> MKHHHHHHMKQNSPLDEENLTQENQDRGTHVDRGLASANVDFAFSLYKQLVLKAPDKNVIFSPLSISTALAFLSLGAHNTTLTEILKGLKFNLTETSEAEIHQSFQHLLRTLNQSSDELQLSMGNAMFVKEQLSLLDRFTEDAKRLYGSEAFATDFQDSAAAKKLINDYVKNGTRGKITDLIKDLDSQTMMVLVNYIFFKAKFEMPFDPQDTHQSRFYLSKKKYVMVPMMSLHHLTIPYFRDEELSCTVVQLNYTGNASALFILPDQDKMEEVEAMLSQETLSRFFDSLEFREIGELYLPKFSISRDYNLNDILLQLGIEEAFTSKAD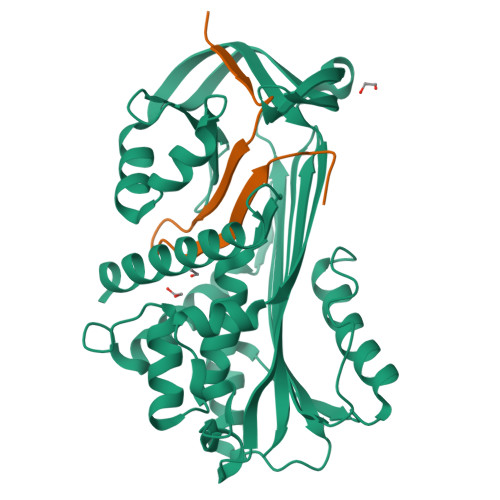LSGITGARNLAVSQVVHKAVLDVFEEGTERSAATALEVLFQ;> GPLVETRTIVRFNRPFLMIIVDHFTWSIFFMSKVTNPKQA> MRGSHHHHHHGSAERAYDFLMPSVNFFGPGVISKIGERAKMLGMKKPVIVTDKFLENLKNGAVAQTLASLKKSGVDYVVYNGVEPNPKIHNIKEVKTLYEKEDADSIITVGGGSAHDTGKGAGIIMTNGDDITKLAGIETLKNPLPPLIAVNTTAGTGSELTRHAVITNEETHLKFVVVSWRNIPLVSFNDPTLMLDIPKGLTAATGMDAFVQAVEPYVSVDHNPITDSQCIQ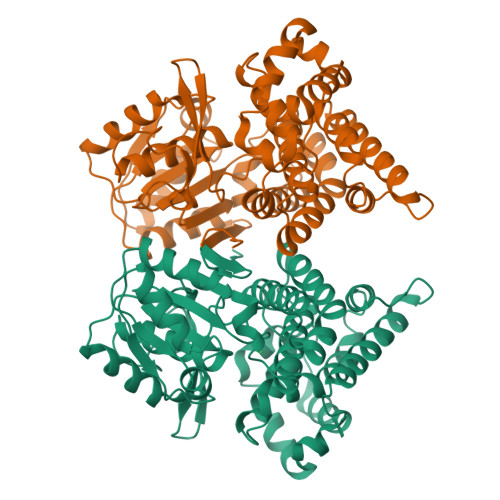AIKLIESSLREAVANGHNLQARTKMVEAEMLAGMAFNNANLGYVHAMAHQLGGQYDAPHGVCCALLLPYAEEYNLIADPERFAELARIMGENTDGLSTRDAAELSIKAMKQLSEDVGIPHSIKDIGAKPEDFDLMAENALKDGNAFSNPRKGTKEDIVKIFQEAYDAK> XSE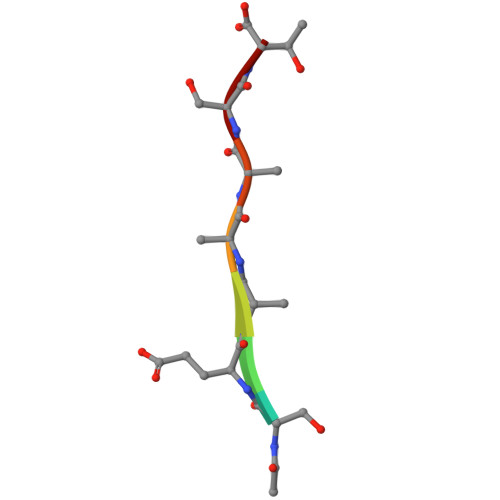AAAST>DN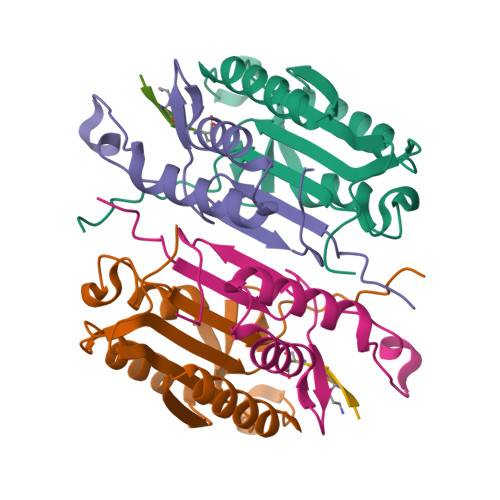SYKMDYPEMGLCIIINNKNFHKSTGMTSRSGTDVDAANLRETFRNLKYEVRNKNDLTREEIVELMRDVSKEDHSKRSSFVCVLLSHGEEGIIFGTNGPVDLKKITNFFRGDRCRSLTGKPKLFIIQACRGTELDCGIET[2x];>[2x]CHKIPVEADFLYAYSTAPGYYSWRNSKDGSWFIQSLCAMLKQYADKLEFMHILTRVNRKVATEFESFSFDATFHAKKQIPCIVSMLTKELYFYHH;>[2x]XVDAVD6'-METHYL-THIAMIN DIPHOSPHATE 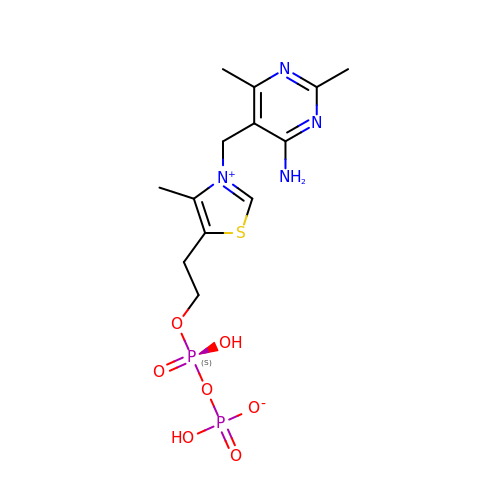| C13 H20 N4 O7 P2 S | XTYXJYCWAJSHCY-UHFFFAOYSA-N> MGSDKIHHHHHHMNTPREVTLHFLRTAGHPLTRWALQRQPPSPKQLEEEFLKIPSNFVSPEDLDIPGHASKDRYKTILPNPQSRVCLGRAQSQEDGDYINANYIRGYDGKEKVYIATQGPMPNTVSDFWEMVWQEEVSLIVMLTQLREGKEKCVHYWPTEEETYGPFQIRIQDMKECPEYTVRQLTIQYQEERRDVKHILFSAWPDH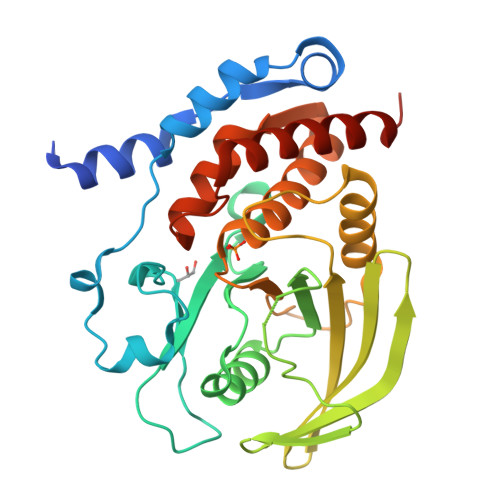QTPESAGPLLRLVAEVEESPETAAHPGPIVVHCSAGIGRTGCFIATRIGCQQLKARGEVDILGIVCQLRLDRGGMIQTAEQYQFLHHTLALYAGQLPEEPSP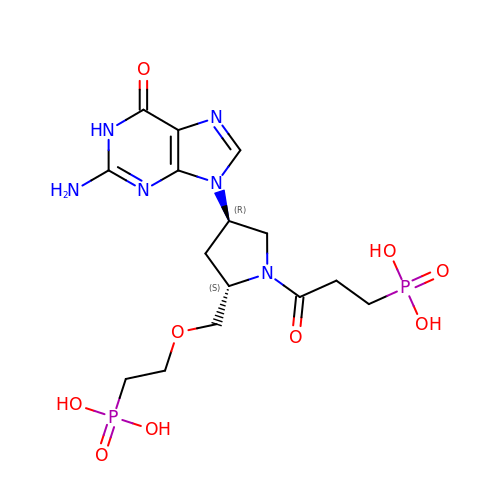(3-{(2S,4R)-4-(2-amino-6-oxo-1,6-dihydro-9H-purin-9-yl)-2-[(2-phosphonoethoxy)methyl]pyrrolidin-1-yl}-3-oxopropyl)phosphonic acid | C15 H24 N6 O9 P2 | APDUDHYPFAMPGN-ZJUUUORDSA-N>[6x]GSSGKRFVHVKNPYLDLMDEDILYHLDLGTKTHNLPAMFGDVKFVCVGGSPNRMKAFALFMHKELGFEEAEEDIKDICAGTDRYCMYKTGPVLAISHGMGIPSISIMLHELIKLLHH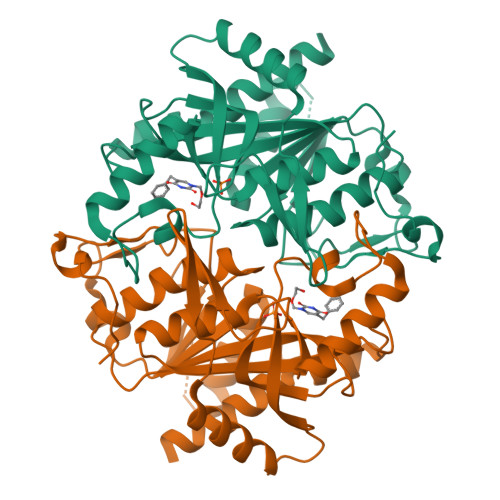ARCCDVTIIRIGTSGGIGIAPGTVVITDIAVDSFFKPRFEQVILDNIVTRSTELDKELSEELFNCSKEIPNFPTLVGHTMCTYDFYEGQGRLDGALCSFSREKKLDYLKRAFKAGVRNIEMESTVFAAMCGLCGLKAAVVCVTLLDRLDCDQINLPHDVLVEYQQRPQLLISNFIRRRLG>GSMFTDWHEAAIGKTHNRMNFDCGDADLNQFLQRHARQNHEKGTTKTYVALDNSDVTRIHGFYSVSPASLIYAQVPGAISKGLGRYDVPVFRLGRLAVDKSMQGQGLGAQLLLSAGKRCIQAALQVGGVALLIDAKNKQVCDWFKGFGAVPLNDQPL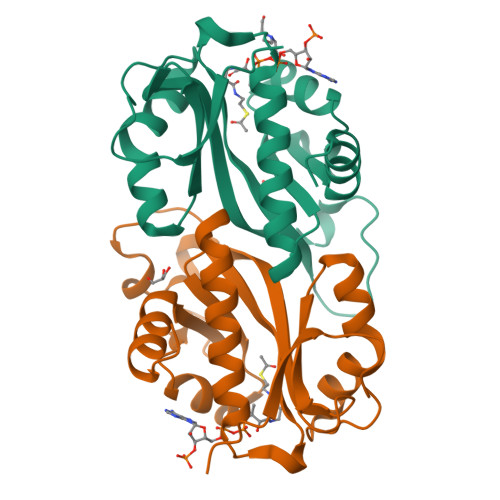SLLLSFKTLYAALSASGRL[2x]> KRFYVKDHRNKAMINLHIQK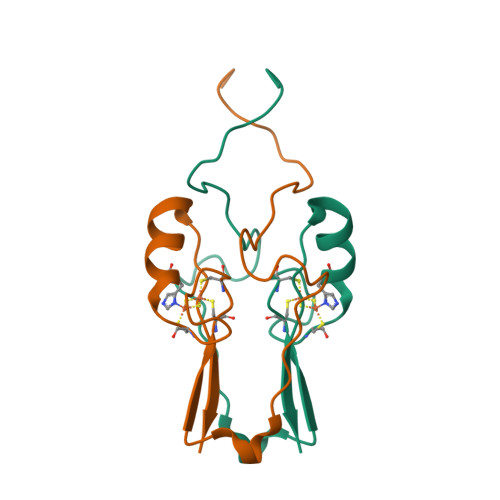DNPKIVHAFDMEDLGDKAVYCRCWRSKKFPFCDGAHTKHNEETGDNVGPLIIKKKETSSGLVPR> GPHMKYKLADYRYGREEMLALFLKDN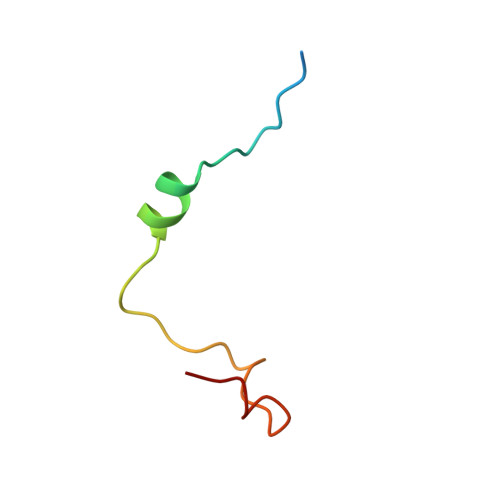KIPSDLLDKEFLPILQ3'-AZIDO-3'-DEOXYTHYMIDINE-5'-DIPHOSPHATE 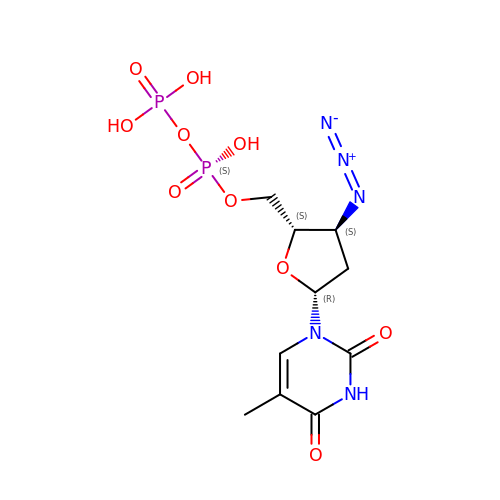| C10 H15 N5 O10 P2 | QOYVAFWJURKBJG-XLPZGREQSA-N> GHMAGGTKRLPRAVREQQMLDAAVDVFSDRGFHETSMDAIAAKAEISKPMLYLYYGSKDELFAACIQREGLRFVEALAPAGDPGLSPREQLRRALEGFLGFVGKHRKSWMVLYRQAMGQQAFV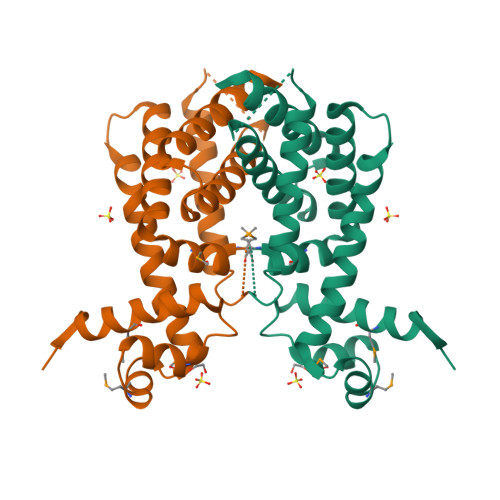GSVQSSRDRLIELTAHLLESSTKDPEPGQDFELIAIALVGAGEAVADRVAGGEIEVDAAADLLESLAWRGLAGKKKPEGS>ACYCRI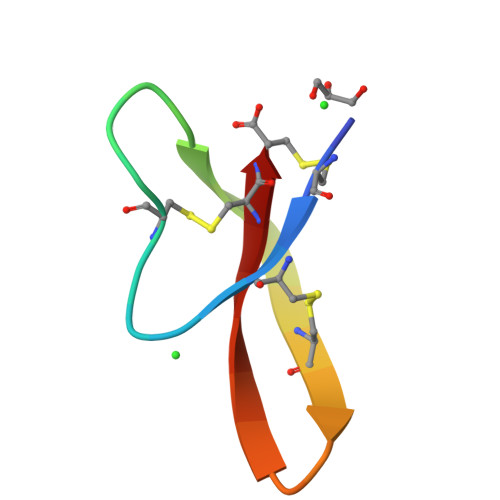PACIAGERRYATCIYQGRLWAFCC[4x]(S)-4-(3-HYDROXYPHENYL)-2-THIOXO-1,2,3,4,7,8-HEXAHYDROQUINAZOLIN-5(6H)-ONE | C14 H14 N2 O2 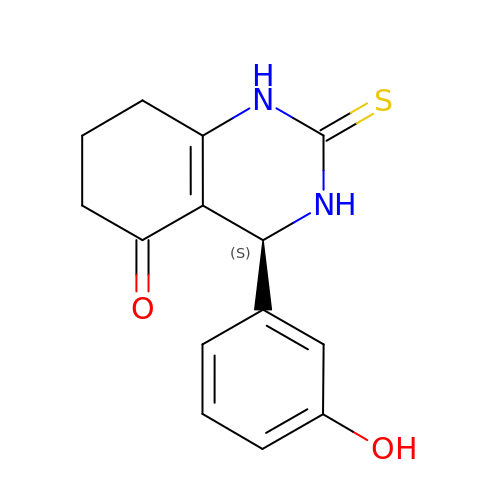S | BJTGVSGWTIUCSM-ZDUSSCGKSA-N>[4x]MFENEILFDNGQHKFMFLGWEEKEEEIVQTNQYLILDGNEGILLDPGGAHVFPRVMSNVAEVVDLSSIRHIFYTHQDPDVTSGILLWLSICENAKIYISSLWVRFLPHFGIYDQKRIVPISDKGTKIKLLSGNEL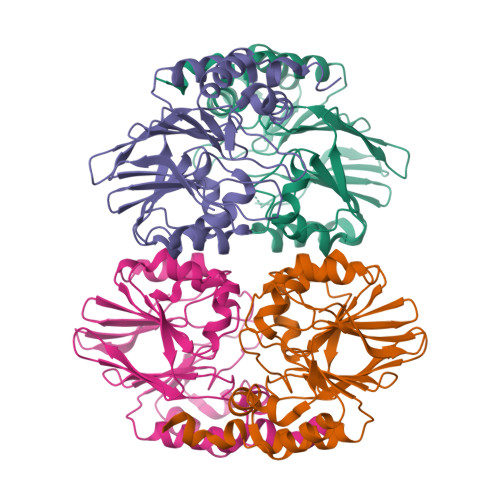EILPAHFLHSTGNFVLYDPVAKILFSGDIGAAVFEKGKRYRYVDDFERHLPLMEAFHKRYMSSNAACKKWVDMVSKKKIDMIAPQHGAVFRGESVKKFLEWFRNLKCGVDLIDNLYSL> MILVNRETRVLVQGITGREGQFHTKQMLTYGTKIVAGVTPGKGGMEVLGVPVYDTVKEAVAHHEVDASIIFVPAPAAADAALEAAHAGIPLIVLITEGIPTLDMVRAVEEIKALGSRLIGG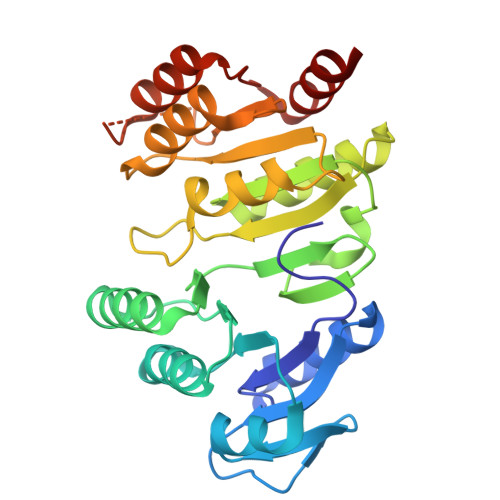NCPGIISAEETKIGIMPGHVFKRGRVGIISRSGTLTYEAAAALSQAGLGTTTTVGIGGDPVIGTTFKDLLPLFNEDPETEAVVLIGEIGGSDEEEAAAWVKDHMKKPVVGFIGGRSAPKGKRMGHAGAIIMGNVGTPESKLRAFAEAGIPVADTIDEIVELVKKALG>[2x]TPQEAQQVDMWKKYIQWEKSNPLRTE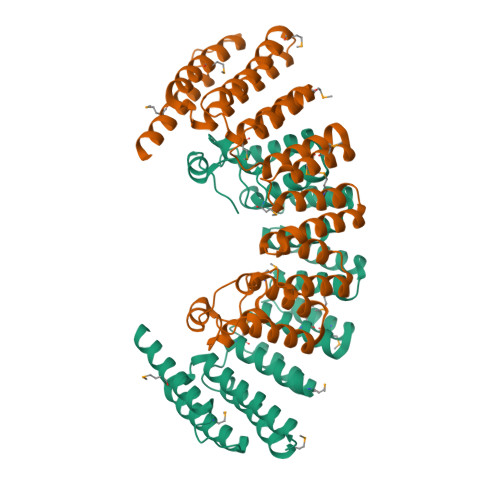DQTLITKRVMFAYEQCLLVLGHHPDIWYEAAQYLEQSSKLLAEKGDMNNAKLFSDEAANIYERAISTLLKKNMLLYFAYADYEESRMKYEKVHSIYNRLLAIEDIDPTLVYIQYMKFARRAEGIKSGRMIFKKAREDARTRHHVYVTAALMEYYCSKDKSVAFKIFELGLKKYGDIPEYVLAYIDYLSHLNEDNNTRVLFERVLTSGSLPPEKSGEIWARFLAFESNIGDLASILKVEKRRFTAFREEYEGKETALLVDRYKFMDLYPCSASELKALGYKDV Phosphoric acid 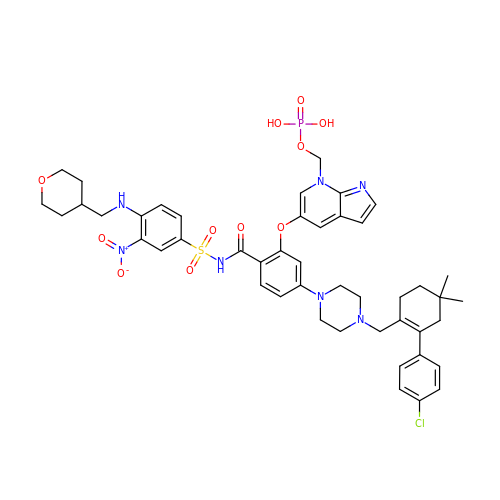mono-[5-(5-{4-[2-(4-chloro-phenyl)-4,4-dimethyl-cyclohex-1-enylmethyl]-piperazin-1-yl}-2-{3-nitro-4-[(tetrahydro-pyran-4-ylmethyl)-amino]-benzenesulfonylaminocarbonyl}-phenoxy)-pyrrolo[2,3-b]pyridin-7-ylmethyl] ester | C46 H53 Cl N7 O11 P S | CLQLTQZFOGFNCT-UHFFFAOYSA-N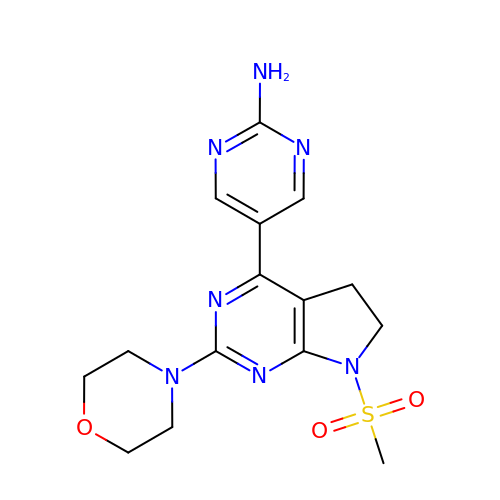5-(7-Methanesulfonyl-2-morpholin-4-yl-6,7-dihydro-5H-pyrrolo[2,3-d]pyrimidin-4-yl)-pyrimidin-2-ylamine | C15 H19 N7 O3 S | JEGHXKRHKHPBJD-UHFFFAOYSA-N> CDLPHTYNLRNKRALKVLAQMRRLPFLSCLKDRQDFGFPLEKVDNQQIQKAQAIPVLRDLTQQTL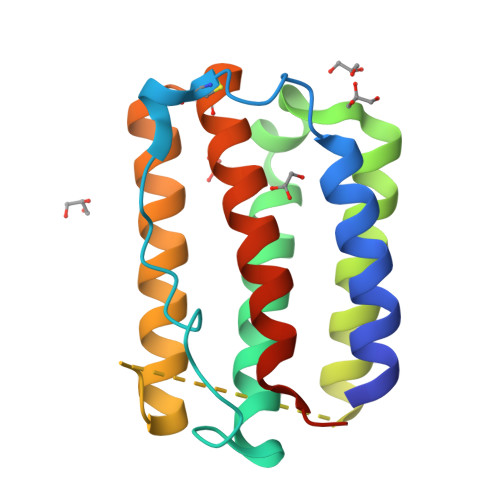NLFTSKASSAAWNTTLLDSFCNDLHQQLNDLQTCLMQQVGVQEPPLTQEDALLAVRKYFHRITVYLREKKHSPCAWEVVRAEVWRALSSSVNLLPRLSEEKE>[4x]MAIDFHLSASQKGTYQAARSLARNLLMPARQTYLQ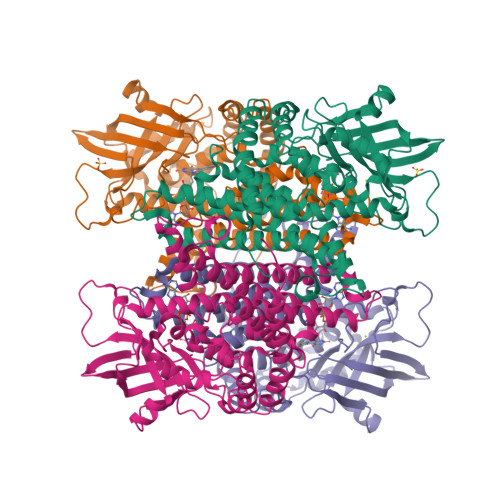HPPNSPLRFQSTQPTYAAAVSAGILKGQISPAHGGTGGTLIESAILVEECYSVEPSAALTIFATGLGLTPINLAAGPQHAEFLAPFLSGEGSPLASLVFSEPGGVANALEKGAPGFQTTARLEGDEWVINGEKMWATNCAGWDFKGCDLACVVCRDATTPLEEGQDPENKVMIILVTRADLDRNGEGSFEVLRHVATPGHTSVSGPHVRYTNVRVPTKNVLCPAGQGAKVAFGAFDGSAVLVGAMGVGLMRAAFDAALKFAKEDNRGGAVPLLERQAFADLLSGVKIQTEAARALTWKAAHAMENGPGDYDARRELALAAKVFCSEAAVKACTDVINAVGISAYDLQRPFSDLLNTAVVLPIFDGGNVGIRRRHLQQLMLKPTYDAWSSTYGSFPGSHHHHHH> MFENITAAPADPILGLADLFRADERPGKINLGIGFYKDETGKTPVLTSVKKAEQYLLENETTKNYLGIDGIPEFGRCTQELLFGKGSALINDKRARTAQTPGGTGALRVAADFLAKNTSVKRVWVSNPSWPNHKSVFNSAGLEVREYAYYDAENHTLDFDALINSLNEAQAGDVVLFHGCCHAPTGIDPTLEQWQTLAQLSVEKGWLPLFDFAYQGFARGLEEDAEGLRAFAAMHKELIVASSYSKNFGLYNERVGACTLVAADSETVDRAFSQMKAAIRANYSNPPAHGASVVATILSNDALRAIWEQELT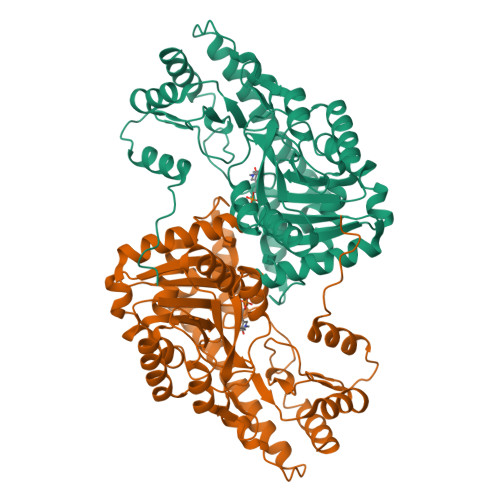DMRQRIQRMRQLFVNTLQEKGANRDFSFIIKQNGMFSFSGLTKEQVLRLREEFGVYAVASGRVNVAGMTPDNMAPLCEAIVAVL> MDECLPNSCLLGVHLVISTHSGPQIVYHYPPSNTAFLTNNPTKHQHLYGNHANLNKNTSTNKEEKLFNSGSTKTASQIALNESAKSYNTAITPSMTNTNTNNVTLPPTRSHANTVGSQSSIPAATNGVGYRKTDIEDTSRTFQYQETESETSSSGLSDSELSTDYLDISSDSFSISSSLSSSSLSSSPSSSSSSSPPQDGLSRTNSSFQSTDSMSPTSPQMIMENDSISVAESYLDSGTNNKSRAASKRSQNFFHKLSTKKSTDSKTHSPVRKLKSKPSQSTKKGNKLLKNTSNETDGNAFTGSCSISSKKSLSSTGEHNQELRNSSLNDTPGQSPHHYHHRYHHYHKNAATSQRNSHTQYDVEEEDMEVSAMLQDGKISMNEIFFEEENFQDINKILEFDNDFVAEFCSPEREMCNTRFEFTVDNFCFLGLPIHVDSQGRWRKSKHKNKTRSKRSSSTTTNISRKKSIASKISSLSENTLKKVNSGEADTVYDSNIGHEASTDTPNLRINTDVSGNEFEREKEDLGKNMNMFHVCFVMNPHLIEYNKRIDDMYQFVVTRLS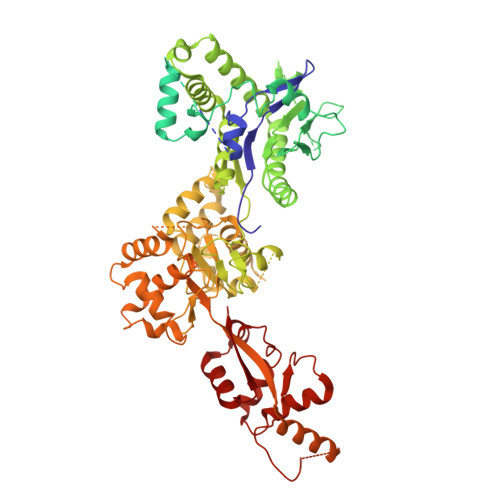LLLRYVQSKTSYISSECHIILKEKERVLKHSKTYQSIRGAGNKGKYLYQRILAKSSLARALTECVDKIQRNEIACLEINDDKVISLQIPIQNEFEKMPNFKLQPVLRGSYLTSILNMKFLEKSSLRIESQNRQNDQAQFSDTNNNIYRFGNNINSTGHCGAANVDDGDDNESNYYCDDNDDLLNYALLLLDEPNNIISSLETFSYQDDIGTIILKHLVRNIQPNIPLRSYRYLITDLLDNPSSLDDLTTETNSLESSILRSCALHLMYWRHARIVIPLSSKYTYIVSPLAPIQGYTIDDYKSTSQNDGNVKKMDDRENNKSGSDRVPLIYQNSMLFRSKFPSLPSLPIFLSLLSTDKPQAYSNIIPSREHKPVYLNALAWLIQYGYVTQLLTFINIRVDKHIKMAVDEDLEKEGFRKTNTARRPSMDYKKTDKKLDDEDGQSRDANASEACSGKNEGMQSNDNNKDVDEKDNENDSRVDDRDDNEIAIADEEEILHFEYDDPEMQHDYTIILEPERATAIEKRWLYRCIYGQPSDIQILFNKLLKYFNGKVPMELVIIKEEISRHDLKKLLNALDKYLIEIHHW> T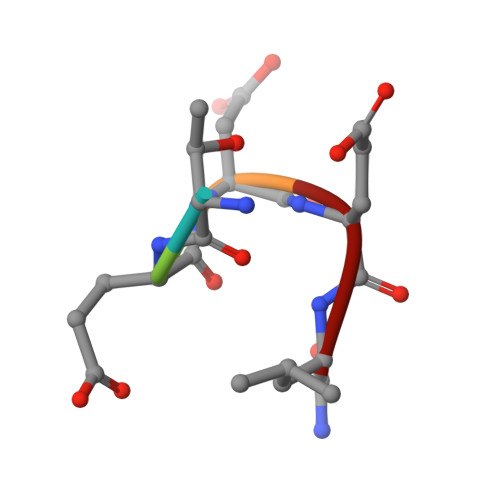EDEL>LGSKRQYADCSEIFNDGYKLSGFYKIKPLQSPAEFSVYCDMSDGGGWTVIQRRSDGSENFNRGWKDYENGFGNFVQKHGEYWLGNKNLHFLTTQEDYTLKIDLADFEKNSRYAQYKNFKVGDEKNFYELNIGEYSGTAGDSLAGNFHPEVQWWASHQR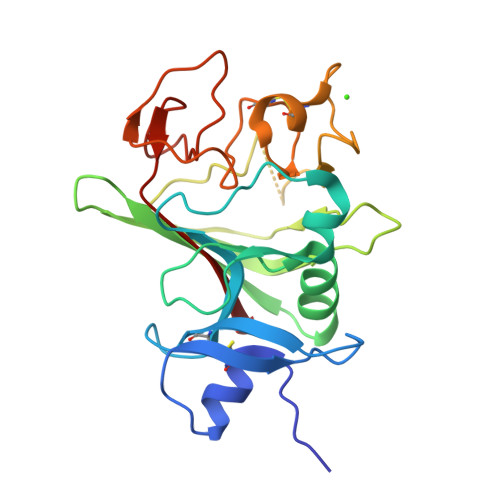MKFSTWDRDHDNYEGNCAEEDQSGWWFNRCHSANLNGVYYSGPYTAKTDNGIVWYTWHGWWYSLKSVVMKIRPND[3x]>GWVIGVDPDIGGAIAVLSPDGSSQVFDNPFVHIVVSEVIRKRLDTKSIIQLLRGLDAPPGTTAYIEKSSPFPTDGKQGWWSTGFSYGLWIASLVASGFSVVPIASQTWKAYFGLMRSETPKDDSRQA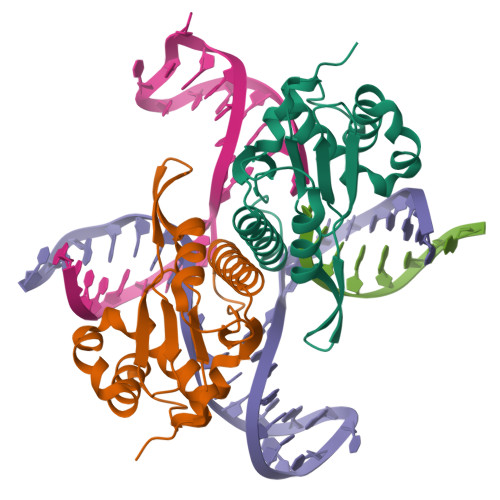ASILFPDKDQSLKLKKHHGRAEALLLAAYGKGLVLP[2x]>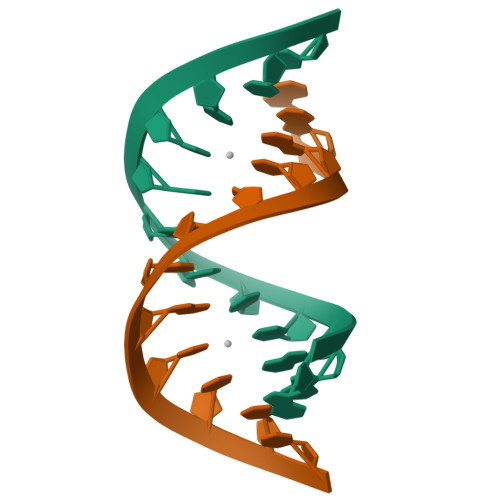GGGCCCGGUCCC[4x]> MKHHHHHHMKQNSPLDEENLTQENQDRGTHVDRGLASANVDFAFSLYKQLVLKAPDKNVIFSPVSISTALAFLSLGAHNTTLTEILKGLKFNLTETSEAEIHQSFQHLLRTLNQSSDELQLSMGNAMFVKEQLSL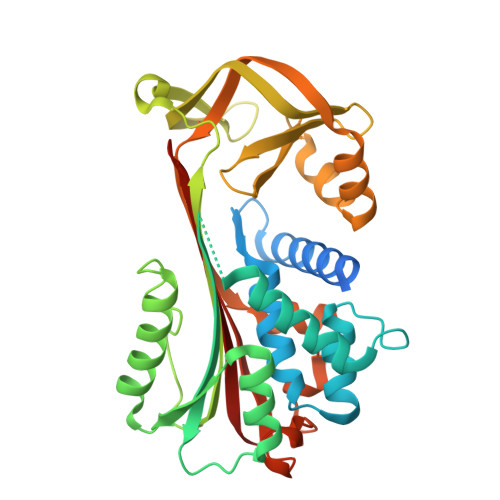LDRFTEDAKRLYGSEAFATDFQDSAAAKKLINDYVKNGTRGKITDLIKDLDSQTMMVLVNYIFFKAKWEMPFDPQDTHQSRFYLSKKKWVMVPMMSLHHLTIPYFRDEELSCTVVQLNYTGNASVFFILPDQDKMEEVEAMLSRETLARWGDSLEFREIGELYLPKFSISRDYNLNDILLQLGIEEAFTSKADLSGITGARNLAVSQVVHKAVLDVFEEGTERSAATAVKITLL>QVPAGTKVTIDGSTSMVNINEALKAQFQQTFPGTVVQTDAQGTDKGVVNLILGKVDLSASSRPLTSQEQAQGLAAVPVASDTIAVMVGRQNPFAGGLTSAQLRDIFTGKISNWSEVGGPNNTIQVINRPSESGTQQ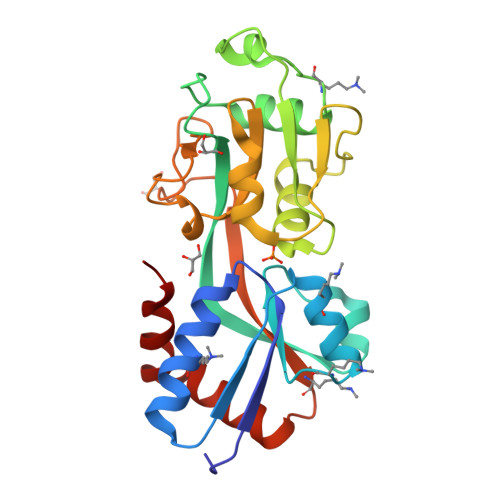TFAAQVLQGQAFGQGANFQTMPRDATTPIIRALGSNGISYATYGQVENQQTARIVPIDSLSPNQENYPLRRQLFYFYKTPPSPQVEAFLGFATSPQGQQAITNAFE[4x]>[2x]MAAQLSEQLAELEKRSGGRVGVIVLDTATGRRIAYRGDERFPMMSTFKALLAAAVLARVDAGKERLGRRITYSKEDLVDYSPVTEKHVGDGMTVAELCEAAITLSDNTAANLLLEALGGPAALTAFLRSIGDEVTRLDRWEPELNEAAPGDERDTTMPAAMAATLRTLLLGDALSPASRQQLVDWLVANKTGGKLLRAGLPADWRI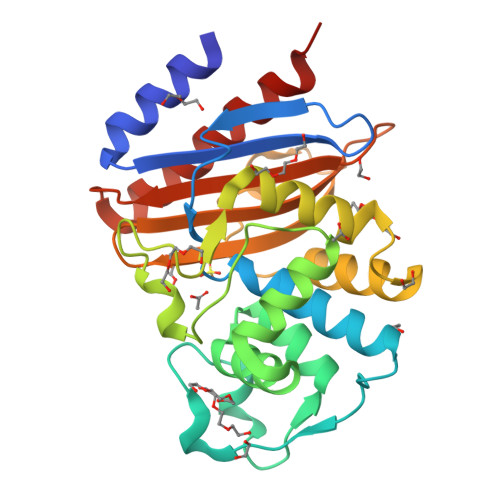GDKSGAGEHGSRNIIAVIGPPGRAPIIVVIYLTESQVDADARDAVIAEVGRLVVEAFHHHHHH> ISEFGSEPIDPSKLE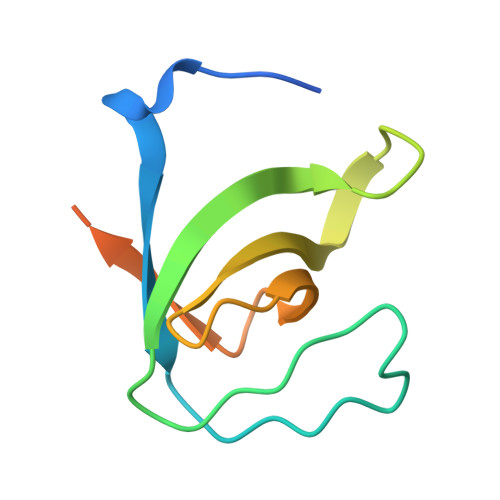FARALYDFVPENPEMEVALKKGDLMAILSKKDPLGRDSDWWKVRTKNGNIGYIPYNYIEIIKRRKKIEHVDDETRTH> MEKTTEGAFYTREYRNLFKEFGYSEAEIQERVKDTWEQLFGDNPETKIYYEVGDDLGYLLDTGNLDVRTEGMSYGMMMAVQMDRKDIFDRIWNWTMKNMYMTEGVHAGYFAWSCQPDGTKNSWGPAPDGEEYFALALFFASHRWGDGDEQPFNYSEQARKLLHTCVHNGEGGPGHPMWNRDNKLIKFIPEVEFSDPSYHLPHFYELFSLWANEEDRVFWKEAAEASREYLKIACHPETGLAPEYAYYDGTPNDEKGYGHFFSSSYRVAANIGLDAEWFGGSEWSAEEINKIQAFFADKEPEDYRRYKIDGEPFEEKSLHPVGLIATNAMGSLA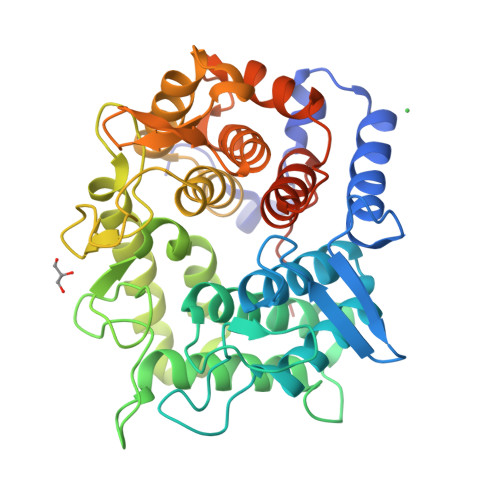SVDGPYAKANVDLFWNTPVRTGNRRYYDNCLYLFAMLALSGNFKIWFPEGQEEEHLEHHHHHH> MSATAATVPP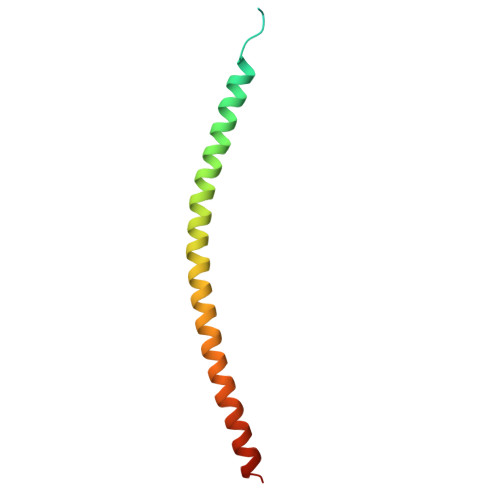AAPAGEGGPPAPPPNLTSNRRLQQTQAQVDEVVDIMRVNVDKVLERDQKLSELDDRADALQAGASQFETSAAKLKRKYWWKNLKMM> ADGIQEAKPSGSVVEQAEGVECDFSPLLSGTPPQVYNFKRLVFTNCNYNLTKLLSLFSVNDFTCSQISPAAIASNCYSSLILDYFSYPLSMKSDLSVSSAGPISQFNYKQSFSNPTCLILATVPHNLTTITKPLKYSYINKCSRLLSDDRTEVPQLVNANQYSPCVSIVPSTVWEDGDYYRKQLSPLEGGGWLVASGSTVAMTEQL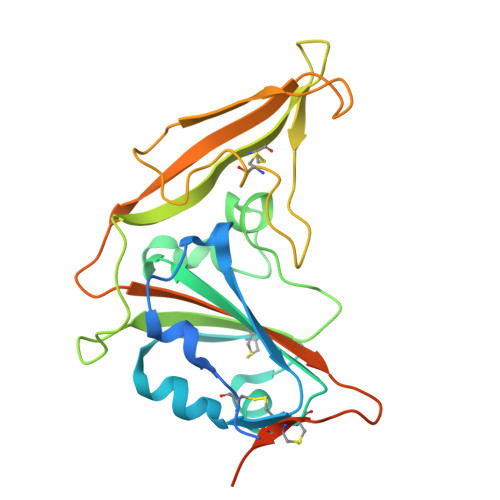QMGFGITVQYGTDTNSVCPKLEFANDTKIASQLGNCVEYHHHHHH> MAMQTSTSSLAKQLFQMTWPMLFGVLSLMSFQLVNSAFIGQLGVLPLAAQGFTMPIQMVIIGIQVGLGIATTAVISRAIGAGKTEYAKQLGGLVIVIG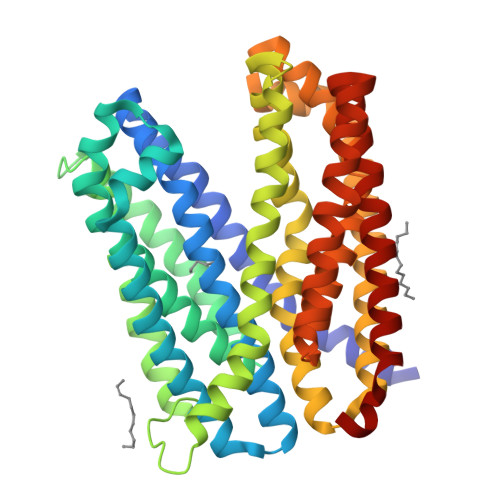GIGVALIALVLYLLRQPLLGLLGAPETVFAIIDHYWLWWLASAWTGAMLYFYYSVCRANGNTLLPGTLMMVTSVLNLILDPIFIFTFDLGIDGAAIATIIAFGVGIAIVAPKVAQRQWTSYQWQDLNISQSLTALGHIMGPAMLSQLLPPLSSMFATKLLASFGTAAVAAWALGSRFEFFALVAVLAMTMSLPPMIGRMLGAKEITHIRQLVRIACQFVLGFQLLIALVTYVFATPLAELMTSETEVSQILNLHLVIVPISLGALGICMLMVSVANALGKSYVALTISALRLFAFYLPCLWLGAHFYGIEGLFIGALVGNIIAGWAAWLAYQKALRSENLYFQ> MREKDYVVIIGSANIDVAGYSHESLNYADSNPGKIKFTPGGVGRNIAQNLALLGNKAWLLSAVGSDFYGQSLLTQTNQSGVYVDKCLIVPGENTSSYLSLLDNTGEMLVAINDMNISNAITAEYLAQHREFIQRAKVIVADCNISEEALAWILDNAANVPVFVDPVSAWKC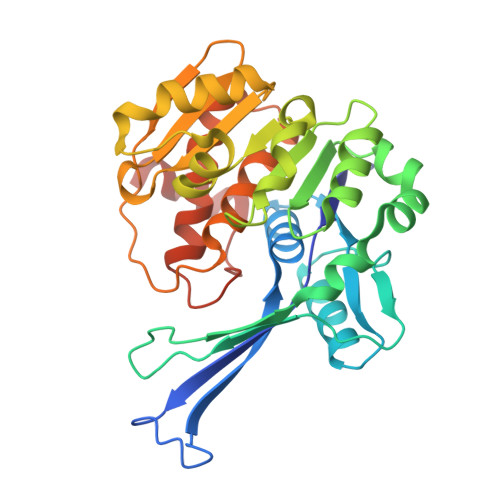VKVRDRLNQIHTLKPNRLEAETLSGIALSGRDDVAKVAAWFHQHGLNRLVLSMGGDGVYYSDIRGENGWSAPIKTNVINVTGAGDAMMAGLASCWVDGMPFAESVRFAQGCSSMALSCEYTNNPDLSIANVISLVENAECLN4-[(4,4-dimethylpiperidin-1-yl)methyl]-2-methylsulfanyl-~{N}-[[(3~{R})-3-oxidanyl-1-[6-[(phenylmethyl)amino]pyrimidin-4-yl]piperidin-3-yl]methyl]benzamide 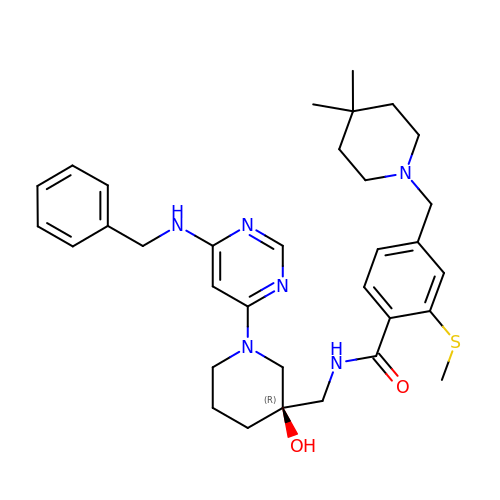| C33 H44 N6 O2 S | CGGPQJWTZLKAFY-MGBGTMOVSA-N> MADDQGCIEEQGVEDSANEDSVDAKPDRSSFVP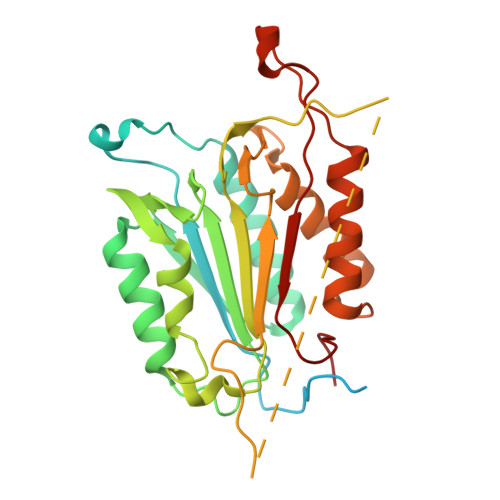SLFSKKKKNVTMRSIKTTRDRVPTYQYNMNFEKLGKCIIINNKNFDKVTGMGVRNGTDKDAEALFKCFRSLGFDVIVYNDCSCAKMQDLLKKASEEDHTNAACFACILLSHGEENVIYGKDGVTPIKDLTAHFRGDRCKTLLEKPKLFFIQAARGTELDDGIQADSGPINDTDANPRYKIPVEADFLFAYSTVPGYYSWRSPGRGSWFVQALCSILEEHGKDLEIMQILTRVNDRVARHFESQSDDPHFHEKKQIPCVVSMLTKELYFSQ> SHPHIQLL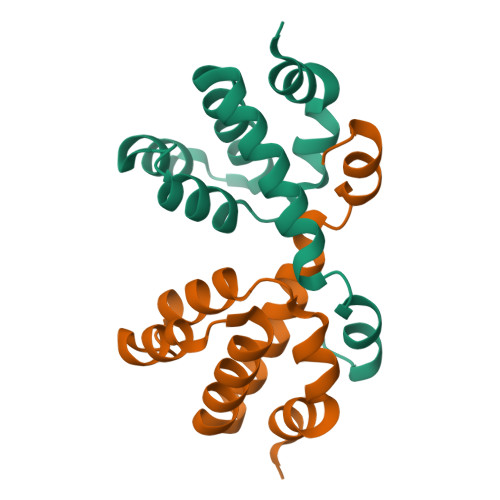KSNRELLVTHIRNTQCLVDNLLKNDYFSAEDAEIVCACPTQPDKVRKILDLVQSKGEEVSEFFLYLLQQLADAYVDLRPWLLEIGLE>[2x]SNAMETFLFTSESVNEGHPDKLCDQVSDAILDACLQQDPESKVACETCTKTNMVMVFGEITTKATVNYEKIVRDTCRGIGFVSADVGLDADNCKVLVNIEQQSPDIAQGVHGHLTKKPEEIGAGDQGHMFGYATDETPELMPLTHVLATKLGAKLTEVRKNKTCAWLRPDGKTQVTVEYQNDNGAMVPIRVHTVLISTQHDETVTNEKIAADLKEHVIKPVIPAKYLDDKTI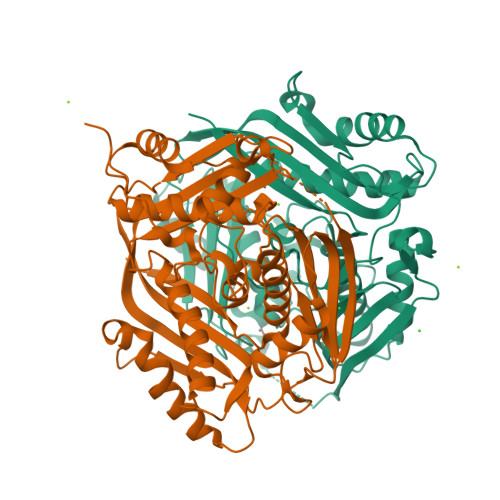FHLNPSGRFVIGGPHGDAGLTGRKIIIDTYGGWGAHGGGAFSGKDPTKVDRSGAYIVRQAAKSVVASGLARRCIVQVSYAIGVPEPLSVFVDTYKTGKIPDKDILVLIKEHFDFRPGMISNNLDLKRGGNFRYQKTAAYGHFGRDDPDFTWETVKILKPKA> MKMYDAYISYVNNENDRKFVNFILKPHLENKYSHKLLLNDTNILPGAEPSAELLMNISRCQRLIVVLSQSYLEQEWCTTNFRQGL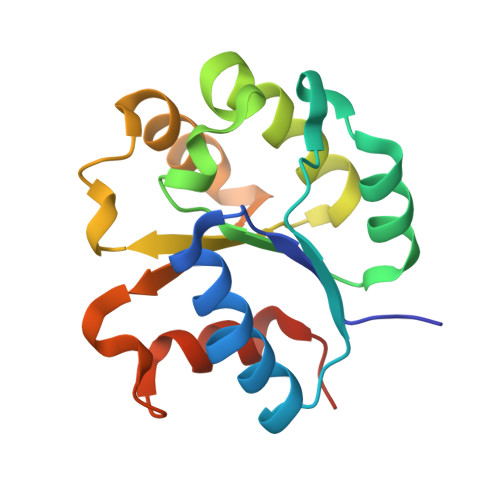WHLIELSRKPIFIIFQSQQKQISQDISQQLRQHQPSITMITWGAHSMTPSSGFWKELALVMPRKHHHHHH>[4x]SEFENPLKRLLVPGEEWEFEVTAFYRGRQVFQQTISCPEGLRLVGSEVGDRTLPGWPVTLPDPGMSLTDRGVMSYVRHVLSCLGGGLALWRAGQWLWAQRLGHCHTYWAVSEELLP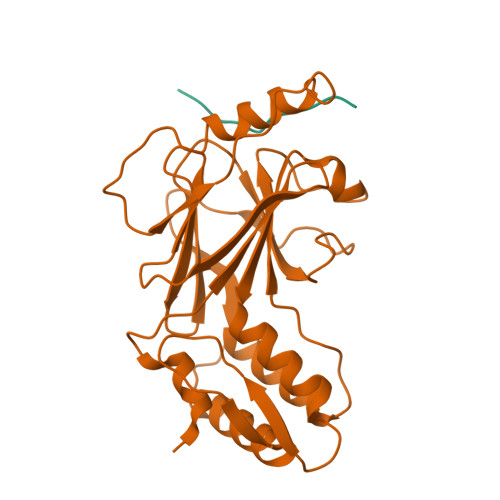NSGHGPDGEVPKDKEGGVFDLGPFIVDLITFTEGSGRSPRYALWFCVGESWPQDQPWTKRLVMVKVVPTCLRALVEMARVGGASSLENTVDLHISNSHPLSLTSDQYKAYLQDLVEGMDFQGPGES;>STLTEEFELLISNSEDDWE[4x]>MQAQLQRPRTTGMLVIMASLMVGTPMAMAAKSSSLDAPQQLQVPTLAYDESSIVLVWKAPEDTRKIVDYQIFSAGKLLGKASDNNDNFSPAKPYIDHFYVNDKDNFQHKIVMQNFTVIGLKPETSYQFTVKAQYADGSLSVASKPITAKTSAKPQIVNVRDFGAIDDGKTLNTKAIQQAIDSCKPGCRVEIPAGTYKSGALWLKSDMTLNLQAGAILLGSENPDDYPAGYRLYPYSTIERPASLINAIDPNNSKPGTFRNIRITGSGVIDGNGWLRAKTAEITDELGRSLPQYVASKNSKVHEDGILAKNQVEKAVSDGMDLKNAYG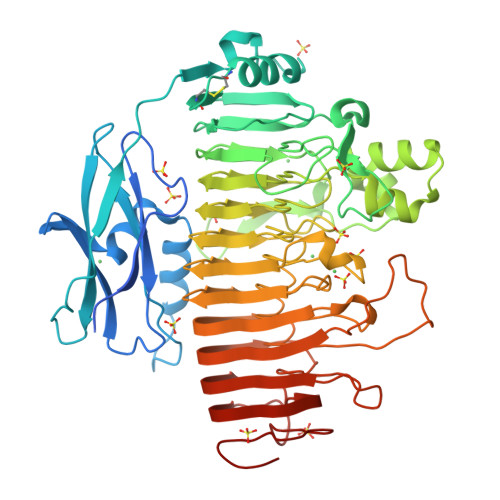QRRSSLMTLRGVENVYLAGFTVRNPAFHGIMNLENHNVVANGLIHQTYDANNGDGIEFGNSQNVMVFNNFFDTGDDCINFAAGTGEKAQEQEPMKGAWLFNNYFRMGHGAIVTGSHTGAWIEDILAENNVMYLTDIGLRAKSTSTIGGGARNVTFRNNAMRDLAKQVMVMTLDYADSNANIDYPPAKIPAQFYDFTLKNVTVDNSTGKNPSIEIKGDTANKAWHRLVHVNNVQLNNVTPTAISDLRDSEFNKVTFTELRGDTPWHFSEVKNVKVDGKPVAP[2x]1-(4-azanyl-3,5,12-triazatetracyclo[9.7.0.0^{2,7}.0^{13,18}]octadeca-1(11),2,4,6,13(18),14,16-heptaen-16-yl)-3-ethyl-pent-1-yn-3-ol 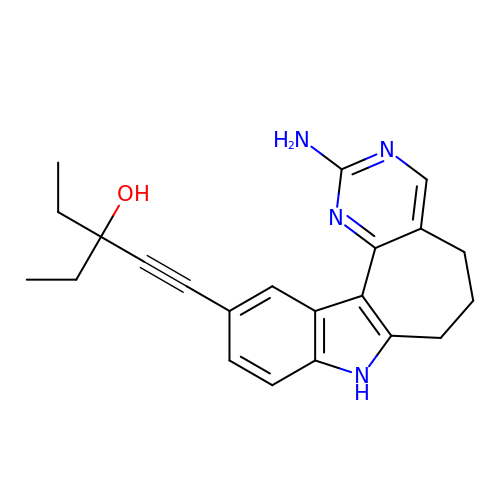| C22 H24 N4 O | HLOKNMXIRZIMSC-UHFFFAOYSA-N4-[(1~{R},5~{S})-6-[2-[4-[3-[[2-[(1~{S})-1-oxidanylethyl]imidazol-1-yl]methyl]-1,2-oxazol-5-yl]phenyl]ethynyl]-3-azabicyclo[3.1.0]hexan-3-yl]butanoic acid | C26 H28 N4 O4 | 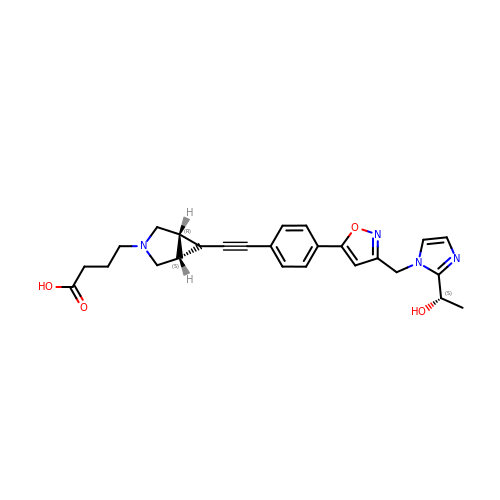PULUMLQUYYSBOR-KEIZBESESA-N>MSPIANGHPHGSSFGVREPKRTGEVSKKMHSKVVIIGSGPGGHTAAIYLARANLEPVLYEGMLANGFAPGGQLTTTTDVENFPGFPEGVTGTEMMDKFRAQSERFGTKIITETVARVDLSVRPFKYWTEGEEEEHEFMTADTIILATGASAKRLFLPGEETYWQSGISACAVCDGAVPIFRQKPLAVIGGGDSAAEEATYLTKYGSHVYVLVRRDELRASKIMAKRLTSHPKVTVLWNTVATEAKGDGEVLTSLTIKNTKTGETGDLPVNGLFYAIGHEPATSLVKSQVELDSDGYIKTVPGTSQTSVHGVFAAGD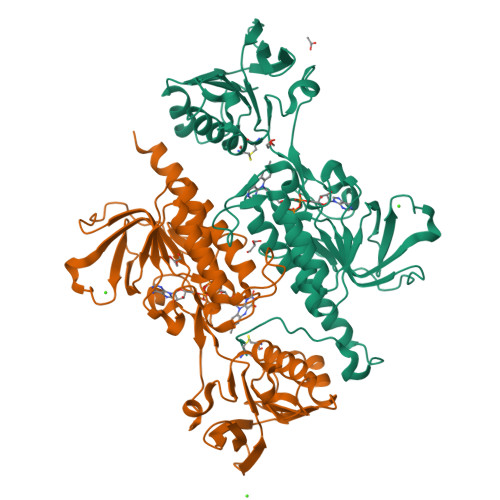VQDKKYRQAITSAGSGCIAALEAERLISEEEADDESLQTEDVHVPAEHYLGTDKE[2x]>[2x]ISEFDSGETMREEQPHLATTWAARGWVEEEGIGSATLGRLVRAWPRRAAVVNKADILDEWADYDTLVPDYPLEIVPFAEHPLFLAAEPHQRQRVLTGMWIGYNERVIATEQLIAEPAFDLVMHGVFPGSDDPLIRKSVQ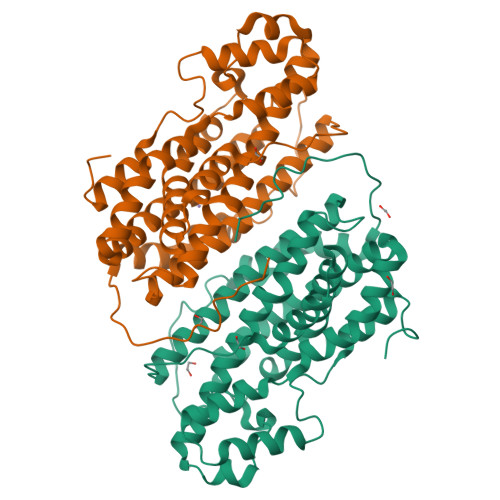QAIVDESFHTYMHMLAIDRTRELRKISERPPQPELVTYRRLRRVLADMPEQWERDIAVLVWGAVAETCINALLALLARDATIQPMHSLITTLHLRDETAHGSIVVEVVRELYARMNEQQRRALVRCLPIALEAFAEQDLSALLLELNAAGIRGAEEIVGDLRSTAGGTRLVRDFSGARKMVEQLGLDDAVDFDFPERPDWSPHTPR>GPMQQANLGDGVATARLLSRSDWGARLPKSVEHFQGPAPYVIIHHSYMPAVCYSTPDCMKSMRDMQDFHQLERGWNDIGFSFGIGGDGMIYTGRGFNVIGAHAPKYNDKSVGIVLIGDWRTELPPKQMLDAAKNLIAFGVFKGYIDPAYKLLGHRQVRDTECPGGRLFAEISSWPHFTHIND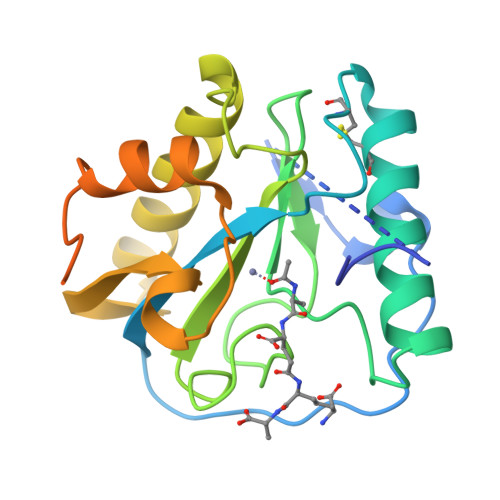TEGVSSTTAPVVPHVHPQAAAPQKPHQSPPAAPKV[2x]> MAVPFVEDWDLVQTLGEGAYGEVQLAVNRVTEEAVAVKIVDMKRAVDCPENIKKEICILKMLNHENVIKFYGHRREGNIQYLFMELASGGSLFDRIEPDIGMPE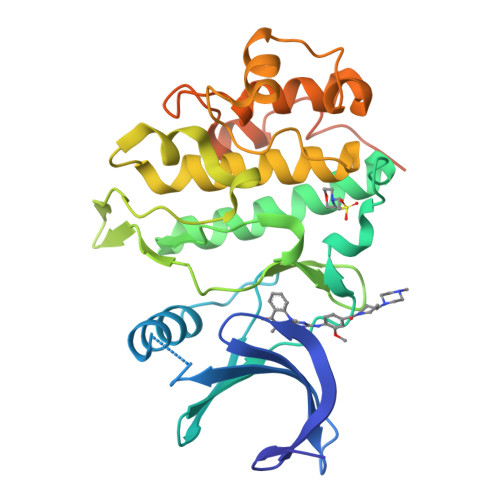PDAQRFFHQLMAGVVYLHGIGITHRDIKPHNLLLDERDNLKIADFGLATVFRYNNRERLLNKMCGTLPYVAPELLKRREFHAEPVDVWSCGIVLTAMLAGELPWDQPSDSCQEYSDWKEKKTYLNPWKKIDSAPLALLHKILVENPSARITIPDIKKDRWYNKPLKKGAKRPRVTSGGVSESPSGHHHHHHHH>[2x]VASLYQAVSLKQEASLFLVGERLNATGSKRFREMLFARDLEGILALAREQVEEGAHALDLSVAWTGRDELEDLRWLLPHLATALTVPVMVDSTSPEAMELALKYLPGRVLLNSANLEDGLERFDRVASLAKAHGAALVVLAIDEKGMAKTREEKVRVALRMYERLTEHHGLRPEDLLFDLLTFPITQGDEESRPLAKETLLAMEELRERLPGVGFVLGVSNV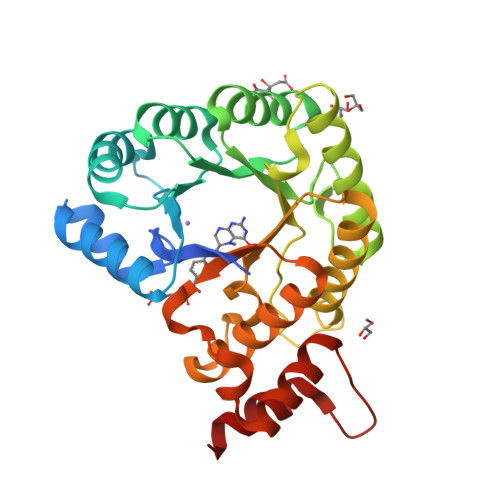SFGLKPRARRVLNSVFLDEARKRGLTAAIVDAGKILPISQIPEEAYALALDLIYDRRKEGFDPLLAFMAYFEAH> GGTIARTIVLQESIGKGRFGEVWRGKWRGEEVAVKIFSSREERSWFREAEIYQTVMLRHENILGFIAADNKDNGTWTQLWLVSDYHEHGSLFDYLNRYTVTVEGMIKLALSTASGLAHLHMEIVGTQGKPAIAHRDLKSKNILVKKNGTCCIADLGLAVRHDSATDTIDIAPNHRVGTKRYMAPEVLDDSINMKHFESFKRADIYAMGLVFWE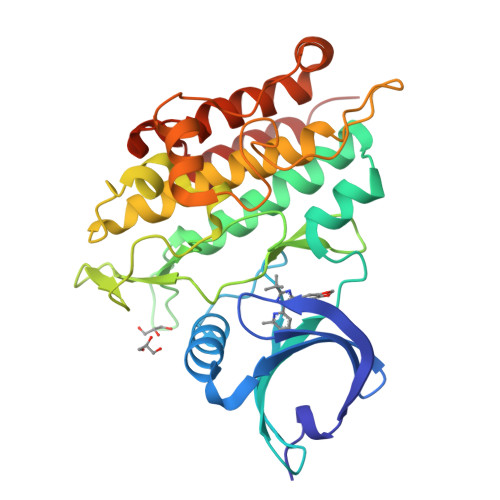IARRCSIGGIHEDYQLPYYDLVPSDPSVEEMRKVVCEQKLRPNIPNRWQSCEALRVMAKIMRECWYANGAARLTALRIKKTLSQLSQQEG>[2x]YKKAGLQRTLVLIKPDAFE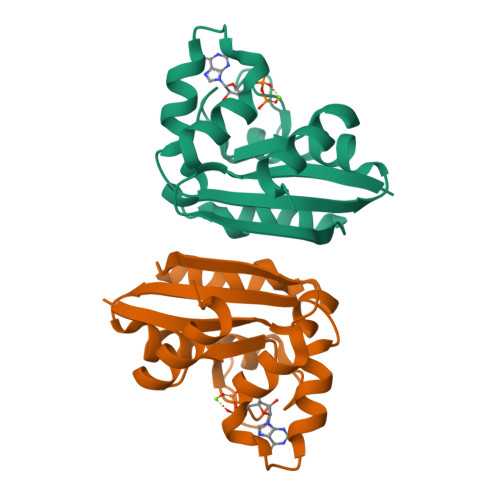RSLVAEIMGRIEKKNFKIVSMKFWSKAPRNLIEQHYKEHSEQSYFNDNCDFMVSGPIISIVYEGTDAISKIRRLQGNTNPLASAPGTIRGDLANDIRENLIHASDSEDSAVDEISIWFPETKMETDN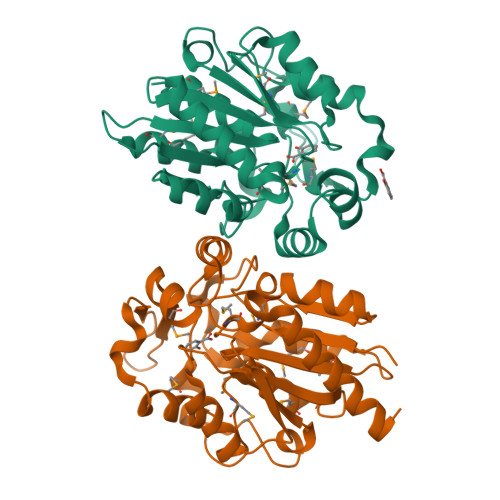>[2x]MKEGKHFVLVHGACHGGWSWYKLKPLLEAAGHKVTALDLAASGTDLRKIEELRTLYDYTLPLMELMESLSADEKVILVGHSLGGMNLGLAMEKYPQKIYAAVFLAAFMPDSVHNSSFVLEQYNERTPAENWLDTQFLPYGSPEEPLTSMFFGPKFLAHKLYQLCSPEDLALASSLVRPSSLFMEDLSKAKYFTDERFGSVKRVYIVCTEDKGIPEEFQRWQIDNIGVTEAIEIKGADHMAMLCEPQKLCASLLEIAHKYNLEHHHHHH> MGKQPVKLKAVVYALSPFQQKIMTGLWK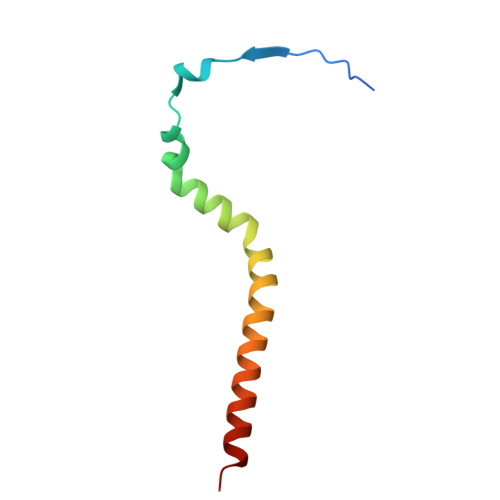DLPEKIHHKVSENWISATLLVTPVVGTYWYAQYFKEQEKLEHRF> MALLLASAINHTAHPAGLRSHPNNESFSRHHLCSSPQNISKRRSNLSFRPRAQTISSESAGIHRLSPWEIPRRDWFPPSFLFGAATSAYQIEGAWNEDGKGPSTWDHFCHNFPEWIVDRSNGDVAADSYHMYAEDVRLLKEMGMDAYRFSISWPRILPKGTLAGGINEKRVEYYNKLIDLLLENGIEPYITIFHWDTPQALVDAYGGFLDERIIKDYTDFAKVCFEKFGKKVKNWLT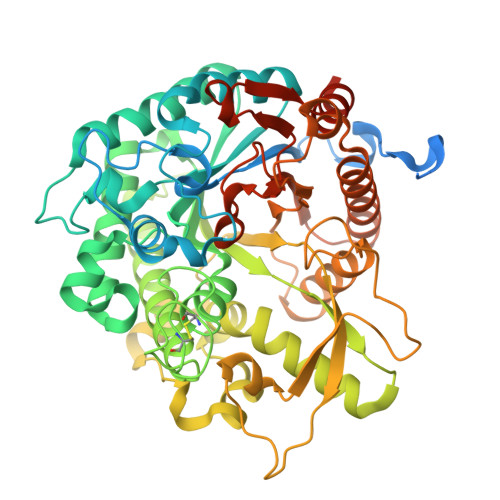FNEPETFCSVSYGTGVLAPGRCSPGVSCAVPTGNSLSEPYIVAHNLLRAHAETVDIYNKYHKGADGRIGLALNVFGRVPYTNTFLDQQAQERSMDKCLGWFLEPVVRGDYPFSMRVSARDRVPYFKEKEQEKLVGSYDMIGINYYTSTFSKHIDLSPNNSPVLNTDDAYASQETKGPDGNAIGPPTGNAWINMYPKGLHDILMTMKNKYGNPPMYITENGMGDIDKGDLPKPVALEDHTRLDYIQRHLSVLKQSIDLGADVRGYFAWSLLDNFEWSSGYTERFGIVYVDRENGCERTMKRSARWLQEFNGAAKKVENNKILTPAGQLN>[2x]SNAEDELYRQSLEIISRYLREQATGAKDTKPMGRSGATSR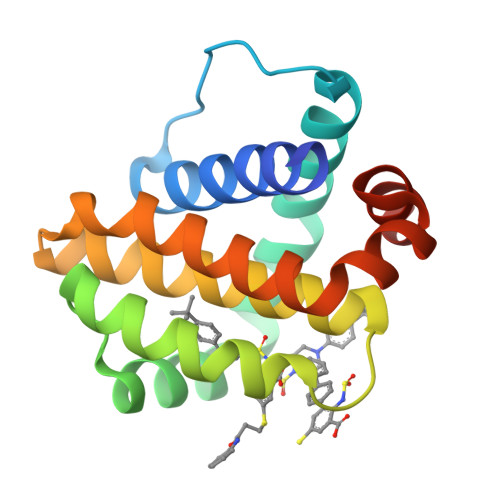KALETLRRVGDGVQRNHETAFQGMLRKLDIKNEDDVKSLSRVMIHVFSDGVTNWGRIVTLISFGAFVAKHLKTINQESCIEPLAESITDVLVRTKRDWLVKQRGWDGFVEFFHVED> MLKKTLAALALGSALFTAGQAMAADYKI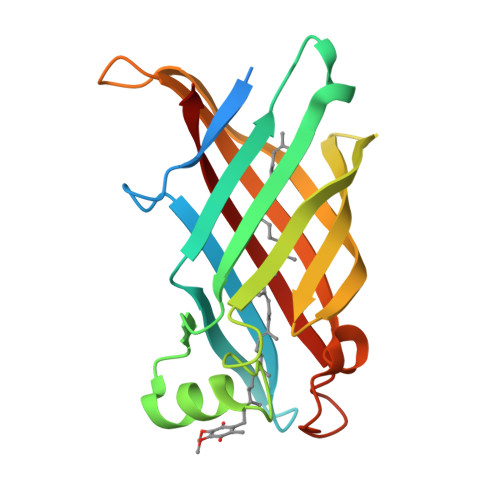DKEGQHAFIEFRIKHLGYSWLYGRFNDFDGSFTFDEKNPSADKVKVTINTNSVDTNHAERDKHLRSGDFLNVSKNPTATFESTEVKANGDSADITGNLTLNGVTKPVTIKAKLIGQGDDPWGGYRAGFEGSATLKLKDFGIKMDLGPASQEVELLLSVEGIRQ>[2x]EVYALEESRDVYLSDLDWLNATHGDDTKSKIVQKNHPFTPGNNNQSTKISLKMEDGSISEFEKGLGTIAGSPSTITYDISGAGVTKFFSYLGID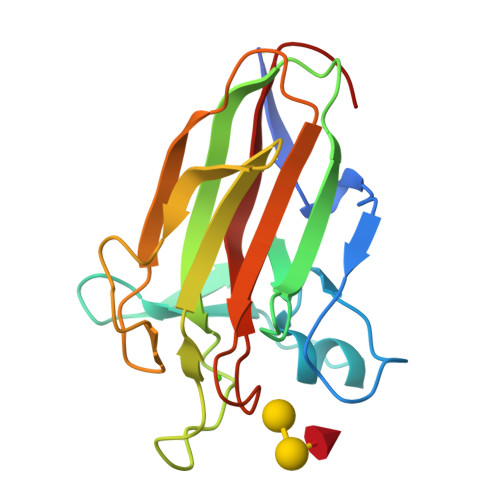RSANPINEQYAKVDKIEVVVDGKVIYSTINQFPNGLTYETPAIKVDLNIPENAKRLQLKSYAGEKTWGDEVVYADAKFTAKGDFVN> MGSSHHHHHHSSGENLYFQGSHMKAIKLTGH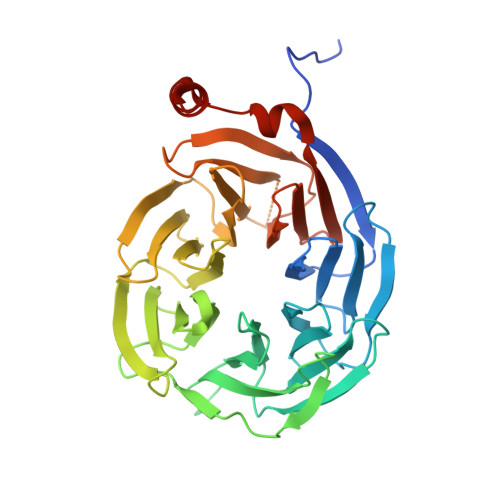ERPLTQVKYNKEGDLLFSCSKDSSASVWYSLNGERLGTLDGHTGTIWSIDVDCFTKYCVTGSADYSIKLWDVSNGQCVATWKSPVPVKRVEFSPCGNYFLAILDNVMKNPGSINIYEIERDSATHELTKVSEEPIHKIITHEGLDAATVAGWSTKGKYIIAGHKDGKISKYDVSNNYEYVDSIDLHEKSISDMQFSPDLTYFITSSRDTNSFLVDVSTLQVLKKYETDCPLNTAVITPLKEFIILGGGQEAKDVTTTSANEGKFEARFYHKIFEEEIGRVQGHFGPLNTVAISPQGTSYASGGEDGFIRLHHFEKSYFDFKYDVEKAAEAKEHMQEAN MuPyV and JCPyV are non-enveloped, circular dsDNA viruses with capsids ~45 nm in diameter. Five copies of VP1 intertwine to form each capsomer subunit that also incorporates one copy of VP2/VP3. The β strands (BIDG and CHEF) are connected by flexible loops (BC, DE, EF, and HI) that extend outward from the surface of the capsomer and comprise the majority of the VP1 hypervariable regions. VP1 C-terminal extensions interact to link capsomers together forming the T = 7 d icosahedron.

The capsomers that occupy the 12 icosahedral fivefold vertices are referred to as pentavalent capsomers, as each of them is surrounded by five neighboring capsomers. The five VP1 molecules within a pentavalent capsomer are structurally identical, whereas the five VP1 molecules within each hexavalent capsomer are quasi-equivalent. To investigate how V296F conferred resistance to 8A7H5, we collected cryo-EM data for purified A2 capsids and A2 capsids incubated with saturating amounts of Fab. Refinement of both datasets produced maps at 3.9 Å and 4.2 Å resolution for the A2 and A2-Fab complex, respectively (Punjani et al., 2017; Zivanov et al., 2018). After icosahedral refinement, we next proceeded with local sub-particle refinement of the constituent hexavalent and pentavalent capsomers for each dataset. This sub-particle refinement allows each capsomer additional degrees of freedom to move independently of the rigid icosahedral matrix, which compensates for imperfect icosahedral symmetry present in flexible virus capsids. Sub-particle refinement improved the resolution of the pentavalent and hexavalent capsomers for both the A2 and A2-Fab complex (2.9 and 3.2 Å, respectively). For each dataset, the constituent capsomers attained approximately equal resolution. Our implementation of sub-particle refinement allowed the rapid solution of the highest resolution cryo-EM structures of any polyomavirus map to date.

>APKRKSGVSKCETKCTKACPRPAPVPKLLIKGGMEVLDLVTGPDSVTEIEAFLNPRMGQPPTPESLTEGGQYYGWSRGINLATSDTEDSPENNTLPTWSMAKLQLPMLNEDLTCDTLQMWEAVSVKTEVVGSGSLLDVHGFNKPTDTVNTKGISTPVEGSQYHVFAVGGEPLDLQGLVTDARTKYKEEGVVTIKTITKKDMVNKDQVLNPISKAKLDKDGMYPVEIWHPDPAKNENTRYFGNYTGGTTTPPVLQFTNTLTTVLLDENGVGPLCKGEGLYLSCVDIMGWRVTRNYDVHHWRGLPRYFKITLRKRWVKNPYPMASLISSLFNNMLPQVQGQPMEGENTQVEEVRVYDGTEPVPGDPDMTRYVDRFGKTKTVFPGN[5x]>MFKPHVTVACVVHAEGKFLVVEETINGKALWNQPAGHLEADETLVEAAARELWEETGISAQPQHFIRMHQWIAPDKTPFLRFLFAIELEQICPTQPHDSDIDCCRWVSAEEILQASNLRSPLVAESIRCYQSGQRYPLEMIGDFNWPFTKGVI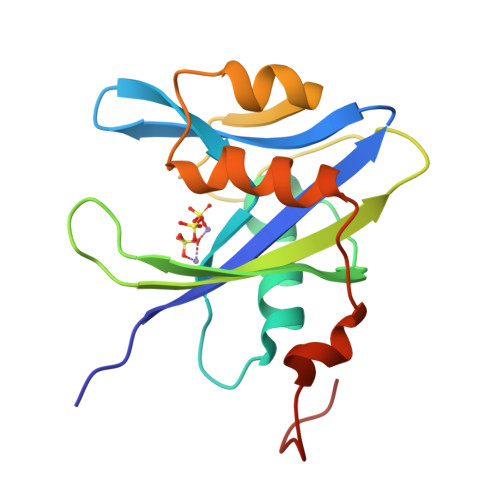[12x]>[2x]MPPYTVVYFPVRGRCAALRMLLADQGQSWKEEVVTVETWQEGS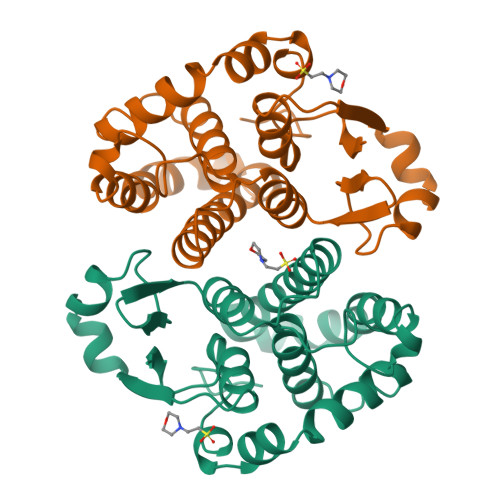LKASCLFGQLPKFQDGDLTLYQSNTILRHLGRTLGLYGKDQQEAALVDMVNDGVEDLRCKYISLIYTNYEAGKDDYVKALPGQLKPFETLLSQNQGGKTFIVGDQISFADYNLLDLLLIHEVLAPGCLDAFPLLSAYVGRLSARPKLKAFLASPEYVNLPINGNGKQ> GMAQAQTQGQEEEQKKKILIVVTHGPEDLDRTYAPL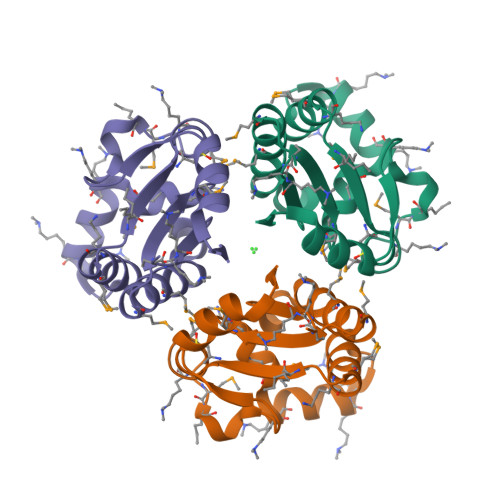FMASISASMEYETSVFFMIKGPKLLDKKWQEEERKKGGNPFIHFFDMAKENGVKMYVCVQSLKDMCHMKEDDVVEGIELVGGSTLIDLTLEADRTLFF>MATRIAILGAGPSGMAQLRAFQSAQEKGAEIPELVCFEKQADWGGQWNYTWRTGLDENGEPVHSSMYRYLWSNGPKECLEFADYTFDEHFGKPIASYPPREVLWDYIKGRVEKAGVRKYIRFNTAVRHVEFNEDSQTFTVTVQDHTTDTIYSEEFDYVVCCTGHFSTPYVPEFEGFEKFGGRILHAHDFRDALEFKDKTVLLVGSSYSAEDIGSQCYKYGAKKLISCYRTAPMGYKWPENWDERPNLVRVDTENAYFADGSSEKVDAIILCTGYIHHFPFLNDDLRLVTNNRLWPLNLYKGVVWEDNPKFFYIGMQDQWYSFNMFDAQAWYARDVIMGRLPLPSKEEMKADSMAWREKELTLVTAEEMYTYQGDYIQNLIDMTDYPSFDIPATNKTFLEWKHHKKENIMTFRDHSYRSLMTGTMAPKHHTPWIDALDDSLEAYLSDK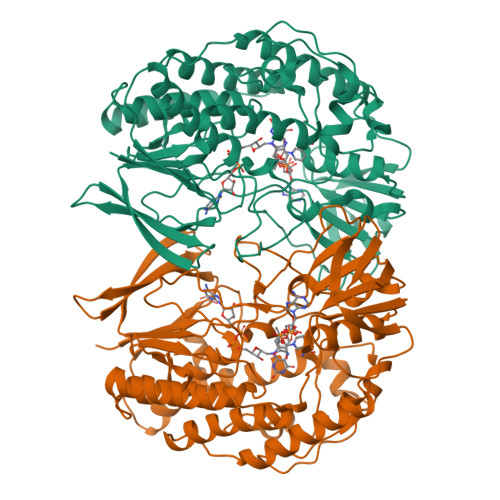SEIPVAKEALEHHHHHH[3x]URIDINE-DIPHOSPHATE-N-ACETYLGLUCOSAMINE 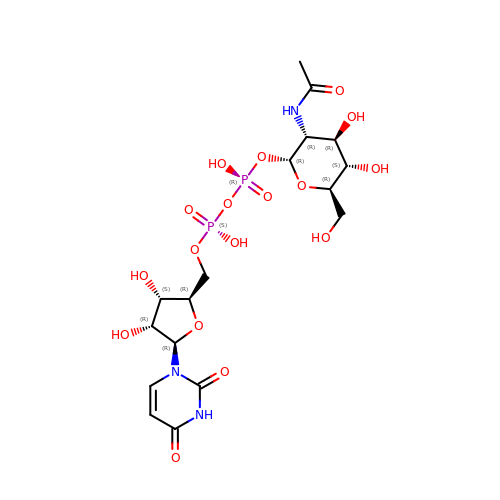| C17 H27 N3 O17 P2 | LFTYTUAZOPRMMI-CFRASDGPSA-N> MHHHHHHAMGKQVSSRGGKSKKLSVTPPSSNGINEELSEVLQTLQDEFGQMSFDHQQLAKLIQESP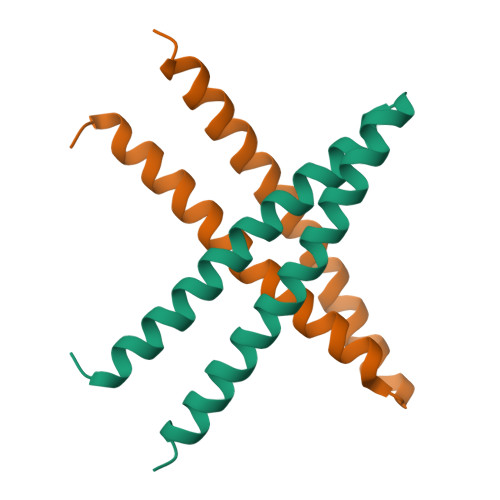TVELKDKLECELEALVGRMEAKANQITKVRKYQAQLEKQKLEKQ> MARKFSSARPEMFRRFTPDSLEEIEAFTELKKSCTLEKKEPESTPRIDLEAGKPLPMIYGDPPEDLLNIPLEDLDPFYKTQKTFIVISKGNIINRFNAERALYIFSPFNPIRRGAIRVFVNSAFNFFIMFTIFSNCIFMTISNPPAWSKIVEYTFTGIYTFEVIVKVLSRGFCIGHFTFLRDPWNWLDFSVVTMTYITEFIDLRNVSALRTFRVLRALKTITIFPGLKTIVRALIESMKQMGDVVILTVFSLAVFTLAGMQLFMGNLRHKCIRWPISNVTLDYESAYNTTFDFTAYIENEENQYFLDGALDALLCGNNSDAGKCPEGYTCMKAGRNPNYGYTNYDNFAWTFLCLFRLMLQDYWENLYQMTLRAAGKSYMVFFIMVIFLGSFYLINLILAVVAMAYEEQNQATLAEAQEKEAEFQRAVEQLRIQQEQINDERKASLASQLTQNQEAEITDDGDDAIKECNGKAFPLANIREPSSVKLSTEEQRSDSKSMDSKHSVDKPSLKHKAASTMSVFTLEDLEAARRPCPPVWYKFAGFVFKWNCCGPWVFLKKWVHFVMMDPFTDLFITLCIILNTLFMSIEHHPMNESFQSLLSAGNLVFTTIFAAEMVLKIIALDPYYYFQQTWNIFDSIIVSLSLLELG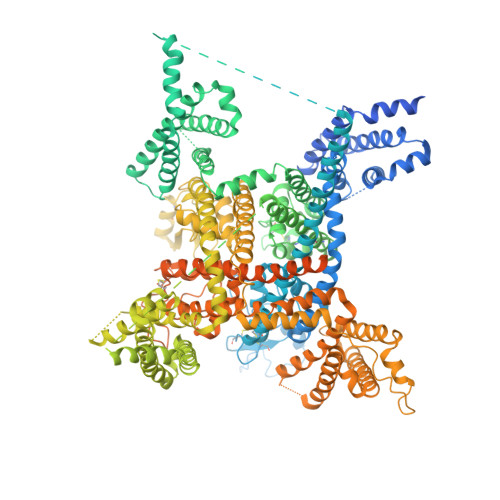LSNMQGMSVLRSLRLLRIFKLAKSWPTLNILIKIICNSVGALGNLTIVLAIIVFIFALVGFQLFGKNYKEYVCKISDDCELPRWHMNDFFHSFLIVFRALCGEWIETMWDCMEVGGVPMCLAVYMMVIIIGNLVMLNLFLALLLSSFSSDNLSSIEEDDEVNSLQVASERISRAKNWVKIFITGTVQALVLWIQGKKPPSDDVVGEEGDNEGKKDTLPLNYLDGEKIVDGITNCVESPTLNLPIVKGESEIEEEGLVDSSDEEDTNKKKHALNDEDSSVCSTVDYSPSEQDPLAKEEEEEEEEEPEELESKDPEACFTEKCIWRFPFLDVDITQGKGKIWWNLRRTCYTIVEHDYFETFIIFMILLSSGVLAFEDIYIWRRRVIKVILEYADKVFTYVFIVEMLLKWVAYGFKRYFTDAWCWLDFVIVGASIMGITSSLLGYEELGAIKNLRTIRALRPLRALSRFEGMKVVVRALLGAIPSIMNVLLVCLMFWLIFSIMGVNLFAGKFYRCINTTTDEILPVEEVNNRSDCMALMYTNEVRWVNLKVNYDNAGMGYLSLLQVSTFKGWMDIMYAAVDSREVEDQPIYEINVYMYLYFVIFIVFGAFFTLNLFIGVIIDNFNRQKQKLGGEDLFMTEEQKKYYNAMKKLGSKKAAKCIPRPSNVVQGVVYDIVTQPFTDIFIMALICINMVAMMVESEDQSQVKKDILSQINVIFVIIFTVECLLKLLALRQYFFTVGWNVFDFAVVVISIIGLLLSDIIEKYFVSPTLFRVIRLARIARVLRLIRAAKGIRTLLFALMMSLPALFNIGLLLFLIMFIFSIFGMSNFAYVKKQGGVDDIFNFETFGNSMICLFEITTSAGWDGLLLPTLNTGPPDCDPDVENPGTDVRGNCGNPGKGITFFCSYIILSFLVVVNMYIAIILENFGVAQEESSDLLCEDDFVMFDETWHKFDVHGTQFLDYNDLPRFVNALQEPMRIPNPNRHKLAKMDMYVVMEDKISYLDVLLAVTQEVLGDTTEMEAMRLSIQAKFKKDNPSPTFFEPVVTTLRRKEEEWASVVIQRAFRQYLLMRAVSHASFLSQIKHMNEGPKDGVGSQDSLITQKMNALYRGNPELTMPLEQQIKPMLDKPRMPSLSVPETYPIQIPKEVTNEVILHSAPMVRQNYSYSGAIVVRESIV> MLVEDLLKNNYLITPSAYYLLSDHYKKAFTLAELIKFAKNRGTFVVDSNLAREFLAEKGIISSGIVYGDYGVPIAYVADETPEEEKAYSTYSDLVIAPKEGFHYRAKEIPDEWELAFDVKNVKFEVPKVKNAQSKEGEVIIQAYSSYFKSRLKKMRRIFRENPEIGTIVDIAKLSYVREDDVTIIGLVNEKRETRKGYLFEIEDATGRIKVFIGSDKEGANEAYSTIMPDSVVAFRGTPGKGIFFANRVFLPDVPKFKRSKPPLEEKVYAILLSDIHVGSNKFCEEAFIKFLEWLNGEVNSRTEEELVSRIKYIIIGGDVVDGVGIYPGQYNELAIPDIFDQYEALANLLKQVPDHITMFIGPGNHDAARTALPQPGFYEEYAKPLYKLKNAVIISNPAVIRLHGRDFLVAHGRGIEDVVDFVPNRSHHRPAEAMVELLKLRHIAPTFGNKVPIAPDPEDTLVIESVPDLFQAGHVHVMQYKTYNGVFVINTGTWQAQTEFQKMVNIIPTPARVPIIDVETARLRAVVRFDQFCEGV;> MSEEIYSPEMKAYFESLQR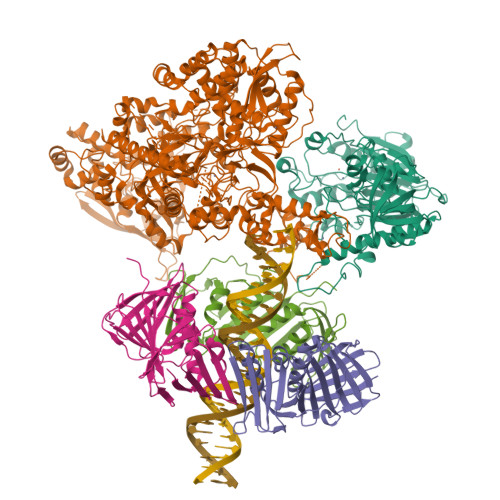EIDRAYAIARKARAQGKDPSFDVEVPQATDMAGRVESLVGPPGVAERIRELVKEYGKEIAALKVVDEIIEGKFGDLGSKEKYAEQAVRTALAILTEGIVSAPLEGIADVKIKRNEWADGSEYLALYYAGPIRSSGGTAQALSVLVGDYVRRKLGLDRFKPSDEHIERMVEEVDLYHRAVTRLQYHPEADEVRLAMRNIPIEITGEETDKVEVSHRNVPGVETNHLRGGAILVLAEGVLQKAKKLVKYIDKMGIEGWDWIKEFVEAKEKGKSSEENKDESKAEDTGTESVAEKKENVEKGFYYELYEKFRANIAPNKKYTKEIIGGRPLFAEPSTNGGFRLRYGRSRVSGFATWSVNPATMLILDEFIAIGTQMKTERPGKGCIVTPATTVEGPIVRLKNGSVVRVDDYETALKVRNEVDEILYVGDALVNFGDFVENNQTLLPANYVEEWWVQELVQAIKDLYEVELQPFAENDREAVEEAAEYLEVDPDFLWNLLKDPLRVKPDVETAIHLSTVLDIPFHPYYTLYWNTLQPEEVEELQKALLGAQIEWAEFRKNRFAKKVVLENDKNIKRYLELLGLPHRLERVEKKRKVIVVEYPWSAALLTPLGNLEWEFKAKPFYTVIDIINENNRIKLRDRGISWIGARMGRPEKAKERKMKPPVQVLFPIGLAGGQSRDIKKAAEEGKTARVEIAFFKCPKCGHVGPEHLCPVCGTRKELLWHCPKCGADYPESDAKDFNYRCPKCDVELKPYAEREIKPADLLRQAMDNVKVYGIDRLKGVKGMTSGYKMAEPLEKGLLRVKNDVYVFKDGTIRFDATDAPITHFKPKEIGTSVEKLRELGYTHDFEGKPLERDDQILELKVQDVILPYEAGRYLLKVARFIDDLLEKFYGLPRFYNAEKMEDLVGHLVIGLAPHTSAGIIGRIIGFSDVLVGYAHPYYHAAKRRNCDGDEDAVMLLLDALLNFSKYYLPEKRGGKMDAPLVVTTRLDPREVDSEVHNMDVVRYYPLEFYKATYELKSPKEVKVIERVEDRLGKPEMYEGIKFTHDTDDIGLGPKMSLYKQLGDMEEKVARQLALAERIRAVDEHHVAETIINSHLVPDLRGNLRSFTRQEFRCVKCNTKYRRPPLTGKCPKCGGKIVLTVSKGAIEKYLPTAKMLVTKYRVKDYTRQRICITEKDIKTLFENVFPEKQRTLMGFSADICEKMVKERTGHSNGKNGYLDEFNGKNGKASKKSGSLASKLSGKGKEPSKKKESAKPKRSEKVKNLTSFEAAAKNEQARGTAGNAKKAESEKPKRKKRKGISLDEFFGS;>MPFEVVFDGAKEFADLIATASNLIDEAAFKFTEEGISMRAMDPSRVVLIDLNLPESIFSKYEVEEPETIGINMDQFKKILKRGKAKDTLILRKGDENFLEITFEGTAKRTFRLPLIDVEELELELPELPFTAKVVLLGEVLKEGIKDASLVSDAIKFIAKENEFTMKAEGETNEVEIRLTLEDEGLLDLEVEEETKSAYGIRYLSDMVKGIGKADEVILRFGNEMPLQMEYMIRDEGRLTFLLAPRVEE[3x]> MSKGKLGEKISQFKIVEELKAKGLYAYFRPIQSKQDTEVKIDGRRVLMFGSNSYLGLTTDTRIIKAAQDALEKYGTGCAGSRFLNGTLDIHVELEEKLSAYVGKEAAILFSTGFQSNLGPLSCLMGRNDYILLDERDHASIIDGSRLSFSKVIKYGHNNMEDLRAKLSRLPEDSAKLICTDGIFSMEGDIVNLPELTSIANEFDAAVMVDDAHSLGVIGHKGAGTASHFGLNDD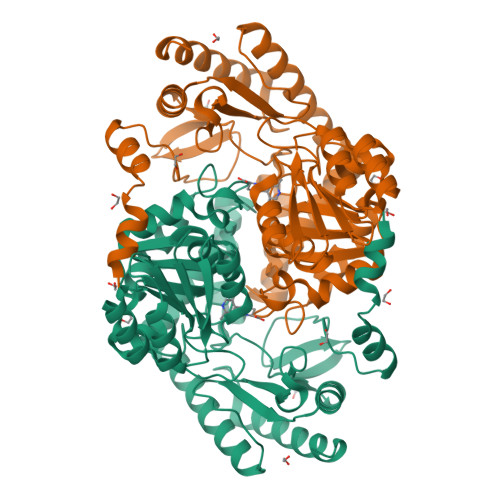VDLIMGTFSKSLASLGGFVAGDADVIDFLKHNARSVMFSASMTPASVASTLKALEIIQNEPEHIEKLWKNTDYAKAQLLDHGFDLGATESPILPIFIRSNEKTFWVTKMLQDDGVFVNPVVSPAVPAEESLIRFSLMATHTYDQIDEAIEKMVKVFKQAEVETLI>[2x]SNAMNELKHLAVVMDGNRRWARAKGFLAKLGYSQGVKTMQKLMEVCMEENISNLSL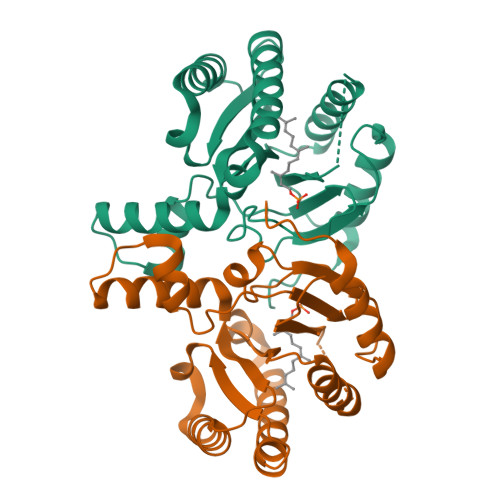FAFSTENWKRPKDEIDFIFELLDRCLDEALEKFEKNNVRLRAIGDLSRLEDKVREKITLVEEKTKHCDALCVNLAISYGARDEIIRAAKRVIEKKLELNEENLTQNLDLPLDVDLMLRVGNAKRLSNFLLWQCSYAEIYFSETLFPSLTKREFKRIIKEFRNRERTFGK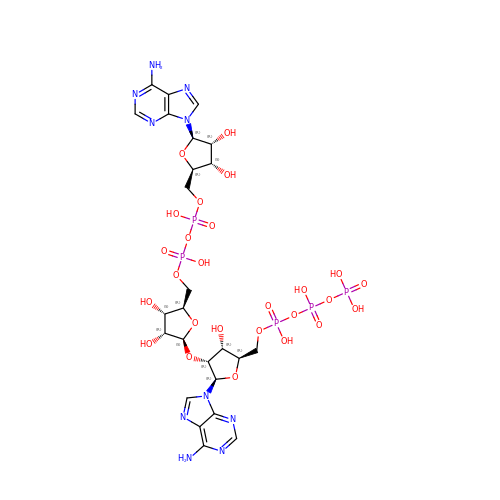[[(2~{R},3~{R},4~{R},5~{R})-5-(6-aminopurin-9-yl)-4-[(2~{S},3~{R},4~{S},5~{R})-5-[[[[(2~{R},3~{S},4~{R},5~{R})-5-(6-aminopurin-9-yl)-3,4-bis(oxidanyl)oxolan-2-yl]methoxy-oxidanyl-phosphoryl]oxy-oxidanyl-phosphoryl]oxymethyl]-3,4-bis(oxidanyl)oxolan-2-yl]oxy-3-oxidanyl-oxolan-2-yl]methoxy-oxidanyl-phosphoryl] phosphono hydrogen phosphate | C25 H37 N10 O26 P5 | BLHBPWIRUPJXKW-VIUUMBSUSA-N> GSMAPRAGFDAEQVRDKARKDLLHLLEGVRGKKNLVIEKDLAGPLGVIVKASTLRDYGVDNFFFLENKNTGTSQRNIVFIARGESVRNAHAIAAQIKRIQRESQTSHDFHIFWVPRRTLFSDKVLEEAGVLGDANISELPLYFFPLERDVLSLELNDSFRDLYLAKDPTPVFLLSRALMGIQKKHGLFPRIIGKGENAKRVADLLSRMRQELLAGEEAGESDRAGLSPSTTIESVIIIDREVDFVTPLLTQLTYEGLIDEYFGIQNNQTDVDAVIVGAPAQSAASTSTAVPTNSSQSRKRKIQLDGSDSLYSQLRDANFAIVGSLLNTVARRLKSDYESRHNTKTTAELKEFV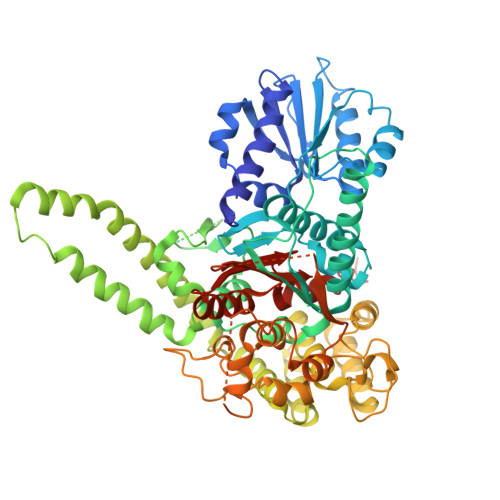KKLPGYQAEQQSLKIHSNIAEEIINYTRTEIFNKLLEVQQNLAAGADPSSQFDSIEELVARDTPLPQVLRLLCLYSCISGGIKTKELDHFRRLVLQGYGHQHLLTLHNLERLQMFLSKSSPLASMITMSGSSGGPDQKTNYTYLRKQLRLIVDEVNEQDPNDIAYVYSGYAPLSIRLVQCVLQKQYLLSITKGSGTVIAAGPVAGGGAQGWKGFEEIVKHARGPTFDEIQKGEDKAVKARALLSGSSGDKKTVFVVFVGGITFTEIAALRFIAKQEEARRNIVICTTSIINGNRMMNAAIETATFEKTTVTTAAAQ> AFAGILADADCAAAVKACEAADSFSYKAFFAKCGLSGKSADDIKKAFVFIDQDKSGFIEEDELKLFLQVFKAGARALTDAETKAFLKAGDSDGDGAIGVEEWVALVKA;> XAFAGILADADCAAAVKAC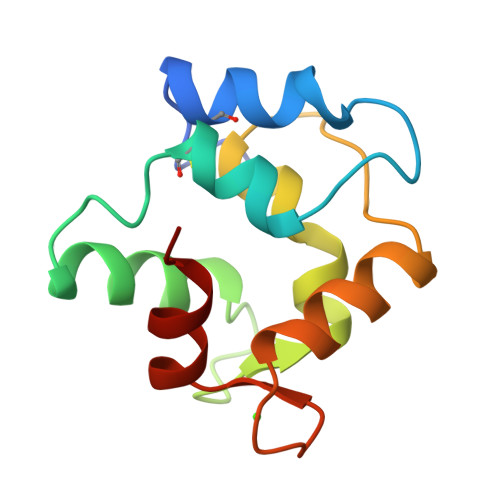EAADSFSYKAFFAKCGLSGKSADDIKKAFVFIDQDKSGFIEEDELKLFLQVFKAGARALTDAETKAFLKAGDSDGDGAIGVEEWVALVKA> RKLSHLRKKLWKEAGPPPDLATRLFSERIMYLGMPIDSSVAELLTAQLFVLVQEAPDPIFFYIN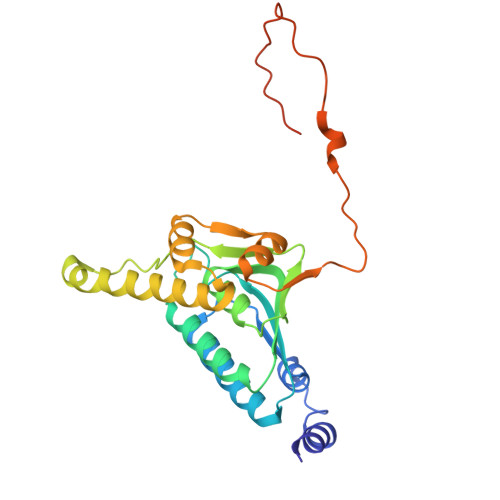STGIAKSTTKFGNEHEAIAVYSMMKGVQKYCPIYTLCVGNAFGEAALLLSAGSPGKRAALRSSTIMLRQPLQRLGGMQASDIDIYRKITREKTATMAKYLAACTKKTEEQIMTDFTRPRYFNPYEAVSYGLIDTVLEPKEERAVFKDWEKMGSEIADLGLWDDEEQPLPTNIMYPGTSQYWRSDFDG> CTGLALETKDGLHLFGRNMDIEYSFNQSIIFIPRNFKCVNKSNKKELTTKYAVLGMGTIFDDYPTFADGMNEKGLGCAGLNFPVYVSYSKEDIEGKTNIPVYNFLLWVLANFSSVEEVKEALKNANIVDIPISENIPNTTLHWMISDITGKSIVVEQTKEKLNVFDNNIGVLTNSPTFDWHVANLNQYVGLRYNQVPEFKLGDQSLTALGQGT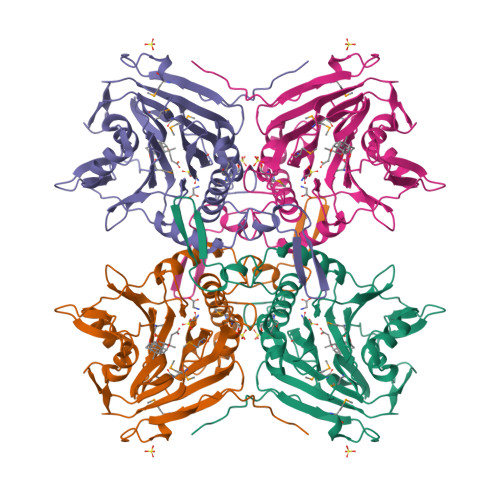GLVGLPGDFTPASRFIRVAFLRDAMIKNDKDSIDLIEFFHILNNVAMVRGSTRTVEEKSDLTQYTSCMCLEKGIYYYNTYENNQINAIDMNKENLDGNEIKTYKYNKTLSINHVN3-methyl-N-[(1R)-1-(5-methyl-1,2-oxazol-3-yl)ethyl]-4-[6-(trifluoromethyl)-1H-indol-3-yl]-1H-pyrrole-2-carboxamide | 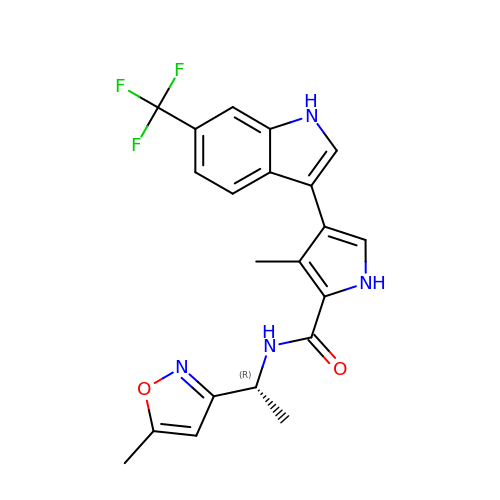C21 H19 F3 N4 O2 | KJKYDILZECXCBA-GFCCVEGCSA-N>SVVLPVAKRGEDILKLIAAPVSANELNSNWLYQLADAMHATMLERNGVGIAAPQVYISKRVIIVASRPNPRYPDAP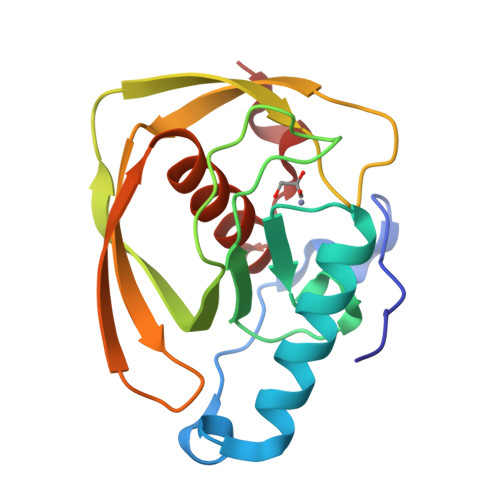EMNAVVMVNPEILEFSSEMCLGEEGCLSVPDERGQVERAEMVKVKYLTLQGEMVETVFQGFPARIVQHEVDHLNGILFVERIS[2x]>TIEKRYDFVFLFDVQDGNPNGDPDAGNLPRIDPQTGEGLVTDVCLKRKVRNFIQMTQNDEHHDIFIREKGILNNLIDEAHEQENVKGKEKGEKTEAARQYMCSRYYDIRTFGAVMTTGKNAGQVRGPVQLTFSRSIDPIMTLEHSITRMAVTNEKDASETGDNRTMGRKFTVPYGLYRCHGFISTHFAKQTGFSENDLELFWQALVNMFDHDHSAARGQMNARGLYVFEHSNNLGDAPADSLFKRIQVVKKDGVEVVRSFDDYLVSVDDKNLEETKLLRKLGG[7x];>GLDRNRQDIGYVLGRLFAVLEKIQAEANPGLNATIADRYFGSASSTPIAVFGTLMRLLPHHLNKLEFEGRAVQLQWEIRQILEHCQRFPNHLNLEQQGLFAIGYYHETQFLFTKDALKNLFNEA[3x];> MILHALTQYYQRKAES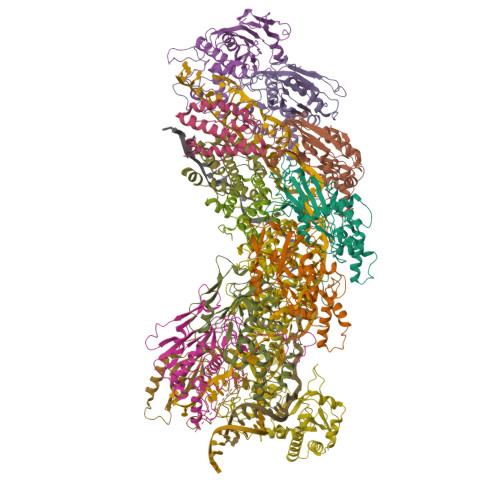DGGIAQEGFENKEIPFIIVIDKQGNFIQLEDTRELKVKKKVGRTFLVPKGLGRSGSKSYEVSNLLWDHYGYVLAYAGEKGQEQADKQHASFTAKVNELKQALPDDAGVTAVAAFLSSAEEKSKVMQAANWAECAKVKGCNLSFRLVDEAVDLVCQSKAVREYVSQANQTQSDNAQKGICLVTGKAAPIARLHNAVKGVNAKPAPFASVNLSAFESYGKEQGFAFPIGEQAMFEYTTALNTLLAGENRFRIGDVTTVCWGAKRTPLEESLASMINGGGKDNPDAHIDAVKALYKSLYNGQYCKPDGEDKFYLLGLSPNSARIVVRFWHETTVAALSESIAAWYDDLQMVRGENSPYPEYMPLPRLLGNLVLDGKMENLPSDLIAQITDAALNNRVLPVSLLQAALRRNKAEQKITYGRASLLKAYINRAIRAGRLKNMKELTMGLDRNRQDIGYVLGRLFAVLEKIQAEANPGLNATIADRYFGSASSTPIAVFGTLMRLLPHHLNKLEFEGRAVQLQWEIRQILEHCQRFPNHLNLEQQGLFAIGYYHETQFLFTKDALKNLFNEA;> RFILEISGDLACFTRSELKVERVSYPVITPSAARNILMAILWKPAIRWKVLKIEILKPIQWTNIRRNEVGTKMSERSGSLYIEDNRQQRASMLLKDVAYRIHADFDMTSEAGESDNYVKFAEMFKRRAKKGQYFHQPYLGCREFPCDFRLLEKAEDGLPLEDITQDFGFMLYDMDFSKSDPRDSNNAEPMFYQCKAVNGVITVPP> GSDVAIVKEGWLHKRGEYIKTWRPRYFLLKNDGTFIGYKERPQDVDQREAPLNNFSVAQCQLMKTERPRPNTFIIRCLQWTTVIERTFHVETPEEREEWTTAIQTVADGLKKQAAAEMDFRSGSPSDNSGAEEMEVSLAKPKHRVTMNEFEYLKLLGKGTFGKVILVKEKATGRYYAMKILKKEVIVAKDEVAHTLTENRVLQNSRHPFLTALKYSFQTHDRLCFVMEYANGGELFFHLSRERVFSEDRARFYGAEIVSALDYLHSEKNVVYRDLKLENLMLDKDGHIKITDFGLCKEGIKDGATMKTFCGTPEYLAPEVLEDNDYGRAVDWWGLGVVMYEMMCGRLPFYNQDHEKLFELILMEEIRFPRTLGPEAKSLLSGLLKKDPKQRLGGGSEDAKEIMQHRFFAGIVWQHVYEKKLSPPFKPQVTSETDTRYFDEEFTAQ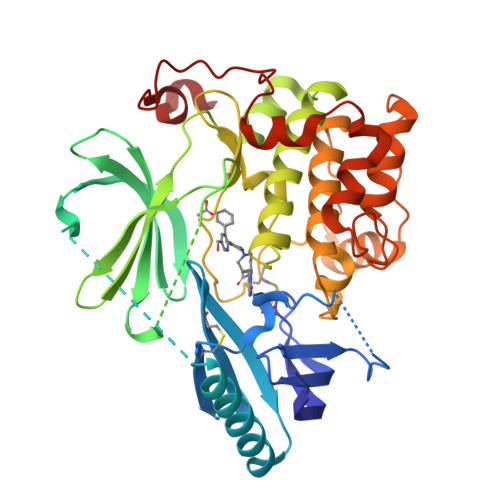M>AMDMTFRYRGPSPKGDQPKAIAGLVEALRDGERFVTLLGATGTGKTVTMAKVIEALGRPALVLAPNKILAAQLAAEFRELFPENAVEYFISYYDYYQPEAYVPGKDLYIEKDASINPEIERLRHSTTRSLLTRRDVIVVASVSAIYGLGDPREYRARNLVVERGKPYPREVLLERLLELGYQRNDIDLSPGRFRAKGEVLEIFPAYETEPIRVELFGDEVERISQVHPVTGERLRELPGFVLFPATHYLSPEGLEEILKEIEKELWERVRYFEERGEVLYAQRLKERTLYDLEMLRVMGTCPGVENYARYFTGKAPGEPPYTLLDYFPEDFLVFLDESHVTVPQLQGMYRGDYARKKTLVDYGFRLPSALDNRPLRFEEFLERVSQVVFVSATPGPFELAHSGRVVEQIIR[2x];>[2x]AMDPPHRPRPGAFRGGERVVHPRFGPGTVVAAQGDEVTVHFEGFGLKRLSLKYAE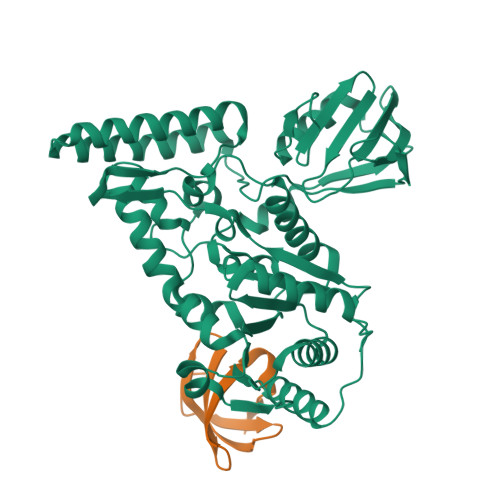LKPA>[2x]AMKKDSKAPCVEVFDERDGCKAAGTQKASGDDGFCVKVSMKAIGFNAAEAASVTKNYGIKRFGAKSV;>[2x]MLDAFSKVITSADGKAAYVGGADLQALKKFVSEGNKRMDSVNAIVSNASCIVSDSVSGMVCENPSLIAPNGGVYTNRKMAACLRDAEIILRYVSYSLLSGDSSVLEDRCLNGLKETYASLGVPAAGNARTISIMKATVIGFITNNSQQKKLSTPAG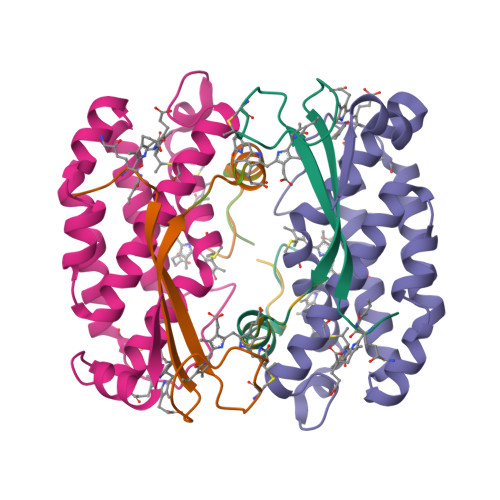DCSALASEVGGYFDKVSSALA;>[2x]AMKKDSKAPCVEVFDERDGCKAAGTQKASGDDGFCVKVSMKAIKMNAAEATSVTKNYNTKLL> MVLGKVVGTVVASRKEPRIEGLSLLLVRAC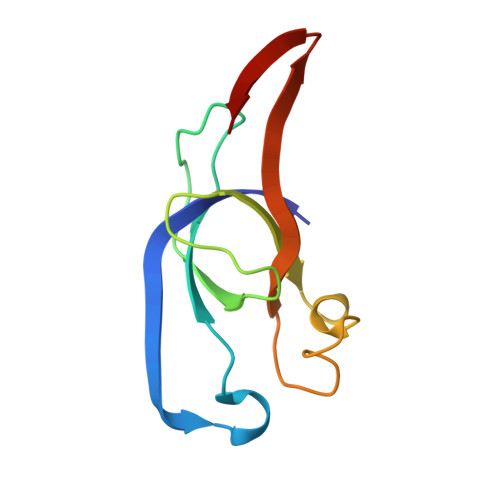DPDGTPTGGAVVCADAVGAGVGEVVLYASGSSARQTEVTNNRPVDATIMAIVDLVEMGGDVRFRKD>[2x]MGSDKIHHHHHHMKKGRGYVYKLEYHLIWATKYRHQVLVDEVADGLKDILRDIATQNGLELVALEVMPDYVHLLLGATPQHVIPDFVKALKGASARRMFSAFPHLKQPHWGGNLWNPSYCVL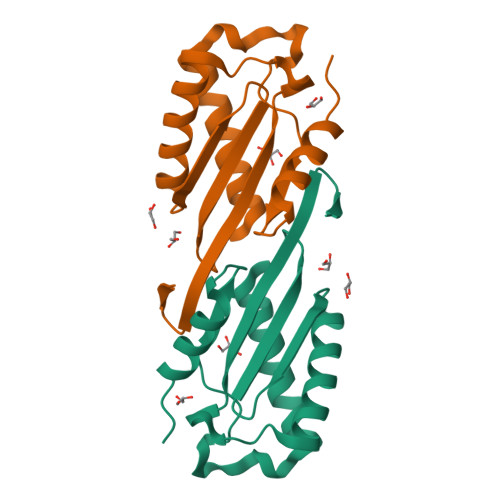TVSEHTRAQIQQYIENQHAAE> MSQNNTISSMNPERAYNNV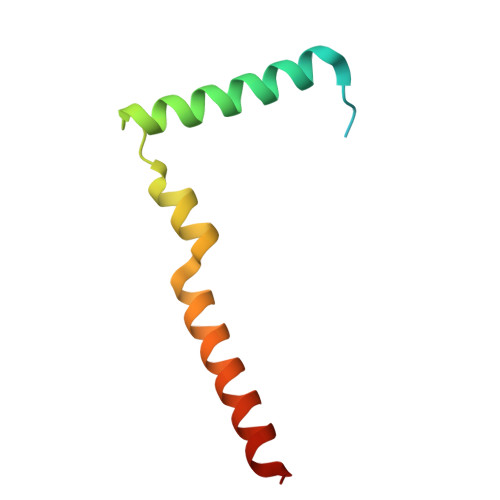TLKNLTAFQLLSQRENICELLNLVESTERHNSIINPERQRMSLEEMKKMLDALKNERKK>[4x]MVALSAEGSSGGSRGGSPKAEAASVPSWPQILGRLTDNRDLARGQAAWAMDQIMTGNARPAQIAAFAVAMTMKAPTADEVGELAGVMLSHAHPLPADTVPDDAVDVVGTGGDGVNTVNLSTMAAIVVAAAGVPVVKHGNRAASSLSGGADTLEALGVRIDLGPDLVARSLAEVGIGFCFAPRF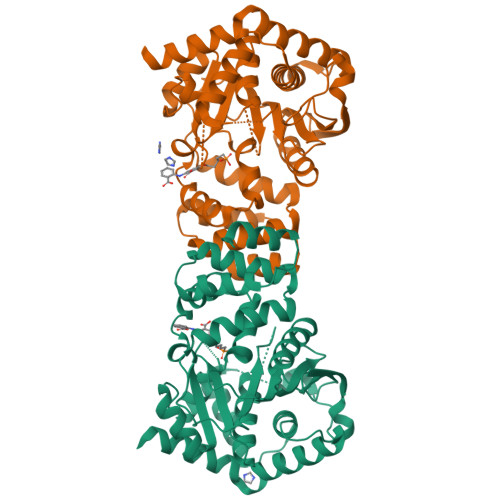HPSYRHAAAVRREIGVPTVFNLLGPLTNPARPRAGLIGCAFADLAEVMAGVFAARRSSVLVVHGDDGLDELTTTTTSTIWRVAAGSVDKLTFDPAGFGFARAQLDQLAGGDAQANAAAVRAVLGGARGPVRDAVVLNAAGAIVAHAGLSSRAEWLPAWEEGLRRASAAIDTGAAEQLLARWVRFGRQILEHHHHHH>[4x]MATQLQQDLTGKVALVTGAASGIGRDIAETYAKAGAAVGIADINLEAAQKTVDAIEAAGGRALAIAMDVTSEAAVNDGVQRLVDTFGGIDILVSNAGIQIIDPIHKMAFEDWKKMLAIHLDGAFLTTKAAIQHMYKDDKGGTVIYMGSVHSHEASLFKAPYVTAKHGLLGLCRVLAKEGAVHNVRSHVICPGFVKTPLVEKQIPQQAAEKGISEESVVNDIMLVNT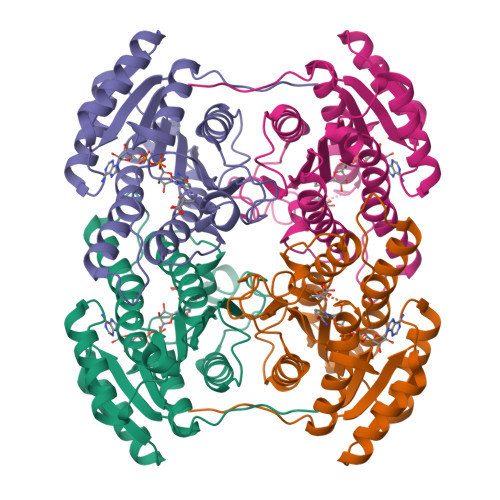VDKEFTTVDDIAQLALFLAAFPTNVFTGQSIVASHGWFMN>SGPKVVIDGKDQNVTGSVVCTTAAGNVNIAIGGAATGIAAVLTDGNPPEVKSVGLGNVNGVTLGYTSGTG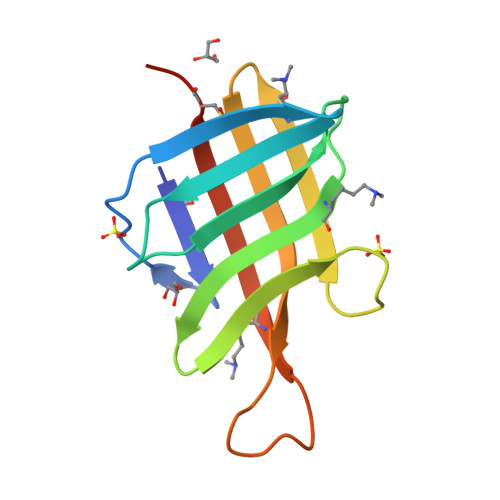QGNASATKDGSHYKITGTATGVDMANPMSPVNKSFEIEVTCSTHHHHHH[7x]> HHHHHHFADLVIQVIDELKQFGVSVKTYGAKGDGVTDDIRAFEKAIESGFPVYVPYGTFMVSRGIKLPSNTVLTGAGKRNAVIRFMDSVGRGESLMYNENVTTGNENIFLSSFTLDGNNKRLGQGISGIGGSRESNLSIRACHNVYIRDIEAVDCTLHGIDITCGGLDYPYLGDGTTAPNPSENIWIENCEATGFGDDGITTHHSQYINILNCYSHDPRLTANCNGFEIDDGSRHVVLSNNRSKGCYGGIEIKAHGDAPAAYNISINGHMSVEDVRSYNFRHIGHHAATAPQSVSAKNIVASNLVSIRPNNKRGFQDNATPRVLAVSAYYGVVINGLTGYTDDPNLLTETVVSVQFRARNCSLNGVVLTGFSNSENGIYVIGGSRGGDAVNISNVTLNNSGRYGVSIGSGIENVSITNISGIGDGINSPVALVSTINSNPEISGLSSIGYPTVARVAGTDYNDGLTLFNGAFRASTTSSGKIHSEGFIMGSTSGCEASVSKSGVLTSSSSKTSSERSLIAGSSTSEAKGTYNTILGSLGAVADEQFAALISASQSRASGNHNLILSSYGINTTGSYKVNGGFEKINWELDSLNGRIKARDTVTGGNTWSDFAQYFESLGGQVIETGYLVTLEKGK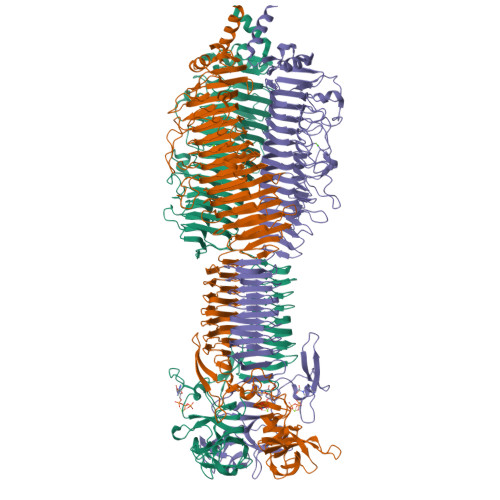IRKAEKGEKIIGVISETAGFVLGESSFEWQGAVLKNEFGGIIYEEVTTEDGVKFKRPLPNPDFDPNKNYIPRSQRREWHVVGLLGQIAVRIDETVKQGHSIDAVGGVATDGDNFIVQEITTPYTKEKGYGVAIVLVK> MENTENSVDSKSIKNLEPKIIHGSESMDSGISLDNSYKMDYPEMGLCIIINNKNFHKSTGMTSRSGTDVDAANLRETFRNLKYEVRNKNDLTREEIVELMRDVSKEDHSKRSSFVCVLLSHGEEGIIFGTNGPVDLKKITNFFRGDRCRSLTGKPKLFIIQACRGTELDCGIETDSGVDDDMACHKIPVEADFLYAYSTAPGYYSWRNSKDGSWFIQSLCAMLKQYADKLEFMHILTRVNRKVATEFESFSFDATFHAKKQI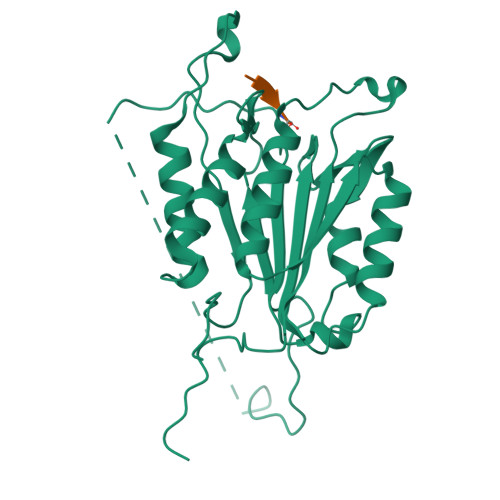PCIVSMLTKELYFYHQLHHHHHH;> XLETD> MGAQVSTQKTGAHETGLNASGNSIIHYTNINYYKDAASNSANRQDFTQDPGKFTEP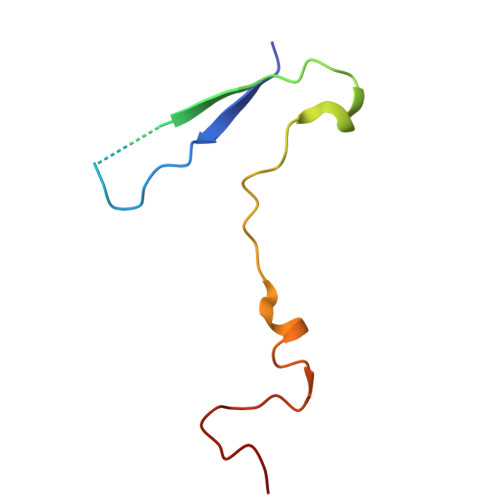VKDIMIKSMPALN> ANNSLEQKAEQVLAPLRLSKEKLQDLSKTFSDELLRGLEMHKRHGLKWVPEECSLRMLDSCVSEIPTGNEKGVFYALDFGGTNVRAVRCELLGGGRIRSQQFLKNLYECGGEIDLMARETSASQLFDVLAGCVGELVEENNEKELLKKKAAKLGFTFSFPCVQRSLNNSVLESWTKGFATGHDTDDPVVGKDVVPLLAAAFARQGLGLECEAVVNDTVGTLLSCAYQKGPGGPPCTVGVILGTGANCCYWEPQAAAFGYRGAVVNVECGNFNKNLPTTPADEAIDNKSPNKKHQLF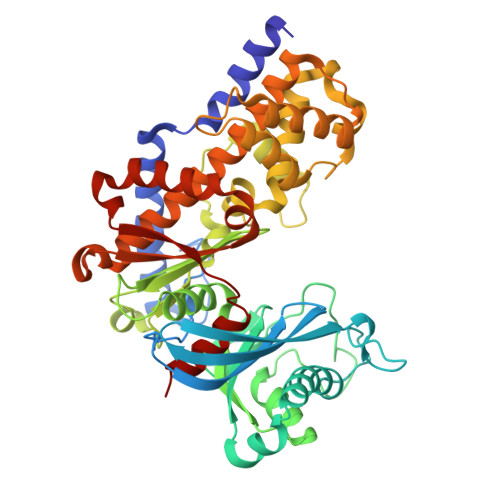EKMISGFYLGELVRLLTLEIFGAAAPAKAREEFSFDAKQAAVLAASLMPGKEEDPALASSCKVLLKESWGWDLDAAALKVMRQIGFAVFDRSAALAAVSIAVLVQRTRSLETDGGVTVAVDGSLYVRNEWYGLRIRTFLKELLGEKVDKVFLRAADDGSGKGAAICVAALH>[2x]DLSQCDREPIHLLGGIQSHGVL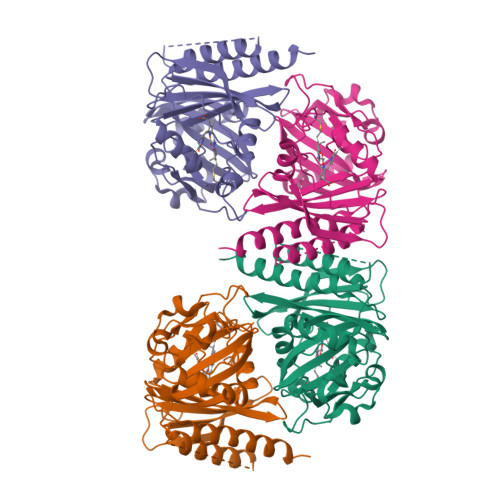LAFRGPDRLLEVVSANAQALLGRPPETLLGQPVGRVLPAEVLAQWEPLVARGSVRVVLPAGAYRALLHESDGLTVLELEPAELQPDMEETALEVVRRLVSPLAGVKGTQALLQTAADTVRALTGFDRVMVYRFDADWHGEVLAESKRGGMDGFLGMHFPATDIPVQARALYTRNPLRLIADARARPVPLLPPVVPALGRPLDLSNSALRSVSPVHLEYLRNMGVGASFSLSLLKEGVLWGLIACHHLEPLHISHERRRACEVLTQLLALQLSAEER>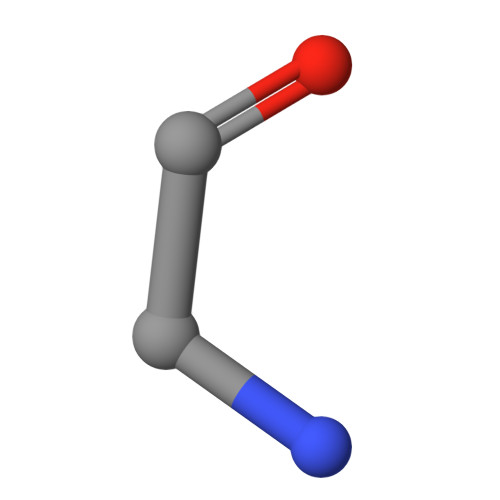 GGGGG> ANKGFLEEVRKGNLERECLEEPCSREEAFEALESLSATDAFWAKY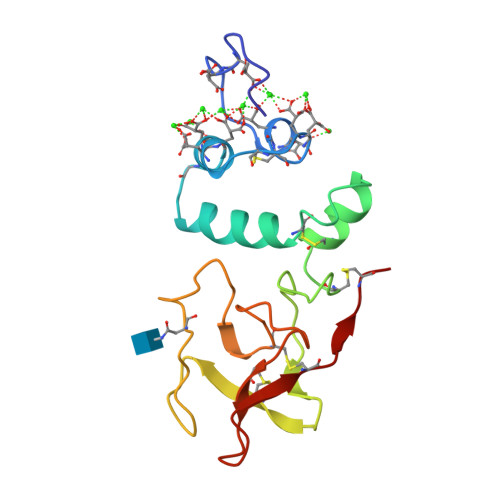TACESARNPREKLNECLEGNCAEGVGMNYRGNVSVTRSGIECQLWRSRYPHKPEINSTTHPGADLRENFCRNPDGSITGPWCYTTSPTLRREECSVPVCG>MSTPGAQQVLFRTGIAAVNSTNHLRVYFQDVYGSIRESLYEGSWANGTEKNVIGNAKLGSPVAATSKELKHIRVYTLTEGNTLQEFAYDSGTGWYNGGLGGAKFQVAPYSCIAAVFLAGTDALQLRIYAQKPDNTIQEYMWNGDGWKEGTNLGGALPGTGIGATS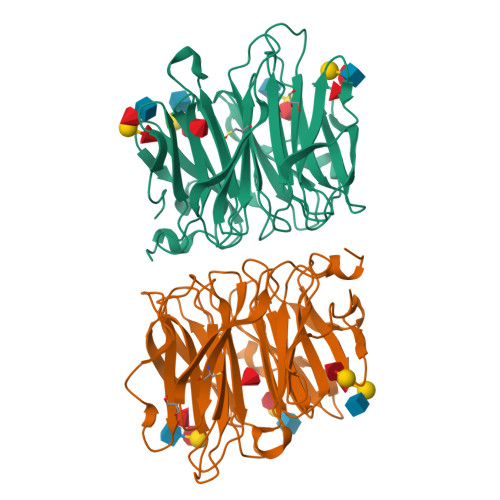FRYTDYNGPSIRIWFQTDDLKLVQRAYDPHKGWYPDLVTIFDRAPPRTAIAATSFGAGNSSIYMRIYFVNSDNTIWQVCWDHGKGYHDKGTITPVIQGSEVAIISWGSFANNGPDLRLYFQNGTYISAVSEWVWNRAHGSQLGRSALPPA[2x]> CAGCAGCCTGAATACCGCA;> GCGGTATTCACCACGAT;> TGCGCTGTGGCTGC;> TCGTGGACAGC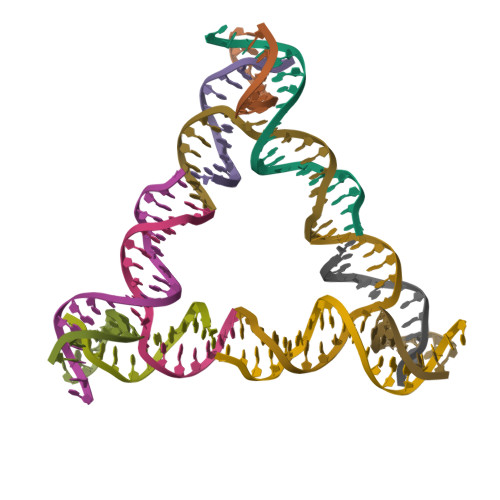G>PVDVSVSIFINKIYGVNTLEQTYKVDGYIVAQWTGKPRKTPGDKPLIVENTQIERWINNGLWVPALEFINVVGSPDTGNKRLMLFPDGRVIYNARFLGSFSNDMDFRLFPFDRQQFVLELEPFSYNNQQLRFSDIQVYTENIDNEEIDEWWIRGKASTHISDIRYDHLSSVQPNQNEFSRITVRIDAVRNPSYYLWSFILPLGLIIAASWSVFWLESFSERLQTSFTLMLTVVAYAFYTSNILPRLPYTTVIDQMIIAGYGSIFAAILLIIFAHHRQANGVEDDLLIQRCRLAFPLGFLAIGCVLVI[5x]

Pentameric ligand-gated ion channels (pLGICs) mediate synaptic transmission and are sensitive to their lipid environment. We demonstrate that the model pLGIC, ELIC (Erwinia ligand-gated ion channel), is positively modulated by the anionic phospholipid, phosphatidylglycerol, from the outer leaflet of the membrane. To investigate the mechanism of positive modulation by POPG, we determined structures of WT ELIC by single particle cryo-electron microscopy (cryo-EM) in the absence and presence of agonist in MSP1E3D1 nanodiscs with 2:1:1 POPC:POPE:POPG (hereafter referred to as 2:1:1) or POPC. In combination with streamlined alchemical free energy perturbation calculations and functional measurements in asymmetric liposomes, the data support a mechanism by which an anionic phospholipid stabilizes the activated, open-channel state of a pLGIC by specific, state-dependent binding to this site.

For all structures, 10 mM cysteamine was used as the agonist since this is a saturating concentration of the most potent, known agonist of ELIC. Likewise, the agonist-bound structures were identical in both lipid conditions, deviating insignificantly from apo and propylamine-bound structures in POPC nanodiscs previously reported. Importantly, the agonist-bound structures showed a non-conducting pore with occlusion at 16’ (F247) and 9’ (L240). Thus, structures of WT ELIC in poorly activating POPC compared to activating 2:1:1 lipids exhibited no meaningful structural differences. Of the six structures obtained in this study, three others show evidence of phospholipid density at this outer leaflet site, including WT apo structures in POPC and 2:1:1, and the WT agonist-bound structure in 2:1:1. Thus, among agonist-bound structures, phospholipid density at this site was not observed in POPC nanodiscs. However, the structures of ELIC in POPC and 2:1:1 nanodiscs from the present study show no differences that point to coupled and uncoupled conformations.>[4x]MGSSHHHHHHSSGLVPRGSHMASATKNASSATPATMTSMVSQRQDLFMTDPLSPGSMFFLPNGAKIFNKLIEFMKLQQKFKFGFNEVVTPLIYKKTLWEKSGHWENYADDMFKVETTDEEKEEYGLKPMNCPGHCLIFGKKDRSYNELPLRFSDFSPLHRNEASGALSGLTRLRKFHQDDGHIFCTPSQVKSEIFNSLKLIDIVYNKIFPFVKGGSGAESNYFINFSTRPDHFIGDLKVWNHAEQVLKE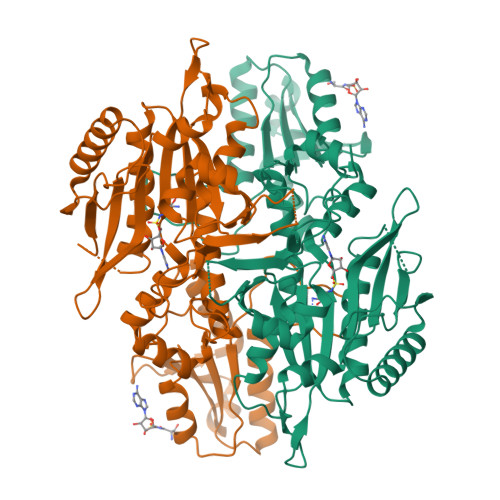ILEESGKPWKLNPGDGAFYGPKLDIMVTDHLRKTHQVATIQLDFQLPERFDLKFKDQDNSYKRPIMIHRATFGSIERFMALLIDSNEGRWPFWLNPYQAVIIPVNTKNVQQLDMCTALQKKLRNELEADDMEPVPLNDWHFNVDLDIRNEPVGYRIKSAILKNYSYLIIVGDEEVQLQKYNIRERDNRKSFEKLTMSQIWEKFIELEKNYK> IRVFAIPPSFASIFLTKSTKLTCLVTDLTTYDSVTISWTRQNGEAVKTHTNISESHPNATFSAVGEASICEDDWNSGERFTCTVTHTDLPSPLKQTISRPKGVALHR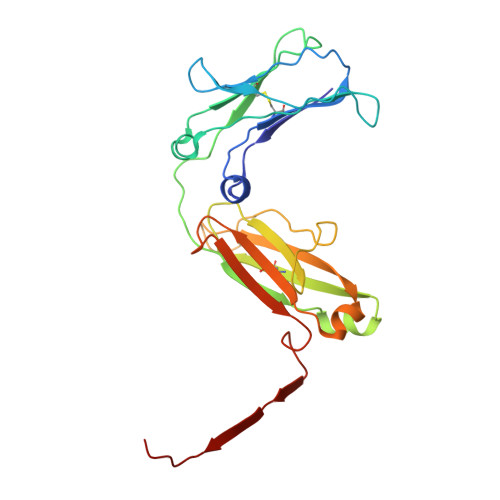PDVYLLPPAREQLNLRESATITCLVTGFSPADVFVQWMQRGQPLSPEKYVTSAPMPEPQAPGRYFAHSILTVSEEEWNTGETYTCVVAHEALPNRVTERTVDKSTGKPTLYNVSLVMSDTAGTCY>[2x]GEFAQECQNLEVERQRRLE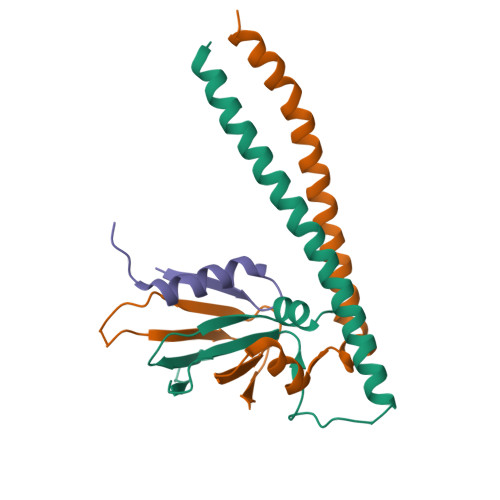RIKQKQSQLQELILQQIAFKNLVQRNRHAEQQASRPPPPNSVIHLPFIIVNTSKKTVIDCSISNDKFEYLFNFDNTFEIHDDIEVLKRMGMACGLESGSCSAEDLKMARSLVPKALEPYVTEMAQGTVGGVFITTA;>GHMKEVIDRLRYLKAEIEDLELKERELDQQKLWLQQSIKNVMDDSINNRFSYVTHEDICNCFNGDTLLAIQAPSGTQLEVPIPEMGQNGQKKYQINLKSHSGPIHVLLINKE[2x];>GEFSGLTPRSALLYKFNGSPSKSLKDINNMIRQGEQRTKKR[2x]> GSVGNREEKILNREIGFAIGMPVCEFDMVKDPEVQDFRRNILNVCKEAVDLRDLNSPHSRAMYVYPPNVESSPELPKHIYNKLDKGQIIVVIWVIVSPNNDKQKYTLKINHDCVPEQVIAEAIRKKTRSMLLSSEQLKLCVLEYQGKYILKVCGCDEYFLEKYPLSQYKYIRSCIMLGRMPNLMLMAKESLYSQLPMDCFTMPSYSRRISTATPYMNGETSTKSLWVINSALRIKILCATYVNVNIRDIDKIYVRTGIYHGGEPLCDNVNTQRVPCSNPRWNEWLNYDIYIPDLPRAARLCLSICSVKGRKGAKEEHCPLAWGNINLFDYTDTLVSGKMALNLWPVPHGLEDLLNPIGVTGSNPNKETPCLELEFDWFSSVVKFPDMSVIEEHANWSVSREAGFSYSHAGLSNRLARDNELRENDKEQLKAISTRDPLSEITEQEKDFLWSHRHYCVTIPEILPKLLLSVKWNSRDEVAQMYCLVKDWPPIKPEQAMELLDCNYPDPMVRGFAVRCLEKYLTDDKLSQYLIQLVQVLKYEQYLDNLLVRFLLKKALTNQRIGHFFFWHLKSEMHNKTVSQRFGLLLESYCRACGMYLKHLNRQVEAMEKLINLTDILKQEKKDET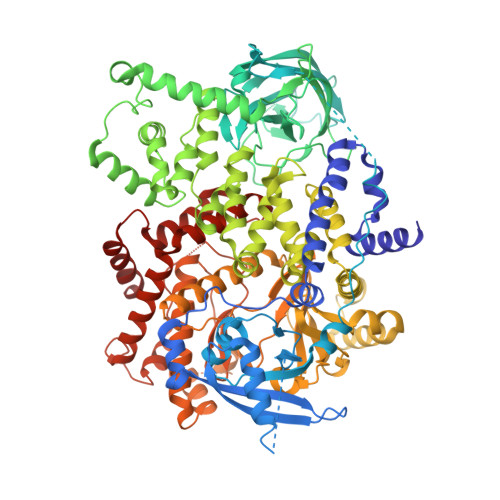QKVQMKFLVEQMRRPDFMDALQGFLSPLNPAHQLGNLRLEECRIMSSAKRPLWLNWENPDIMSELLFQNNEIIFKNGDDLRQDMLTLQIIRIMENIWQNQGLDLRMLPYGCLSIGDCVGLIEVVRNSHTIMQIQCKGGLKGALQFNSHTLHQWLKDKNKGEIYDAAIDLFTRSCAGYCVATFILGIGDRHNSNIMVKDDGQLFHIDFGHFLDHKKKKFGYKRERVPFVLTQDFLIVISKGAQECTKTREFERFQEMCYKAYLAIRQHANLFINLFSMMLGSGMPELQSFDDIAYIRKTLALDKTEQEALEYFMKQMNDAHH>[4x]MSNEIPKPVAPAPDILRCAYAELVVTDLAKSRNFYVDVLGLHVSYEDENQIYLRSFEEFIHHNLVLTKGPVAALKAMAFRVRTPEDVDKAEAYYQELGCR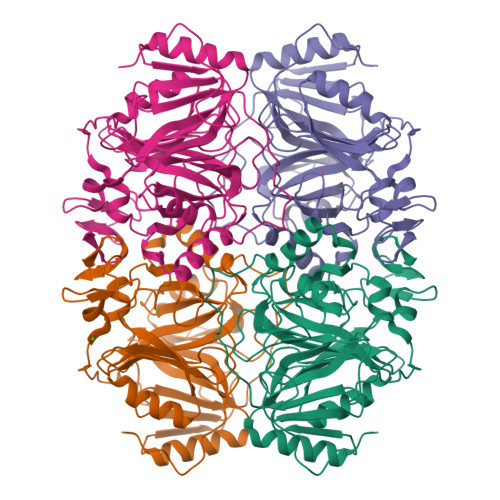TERRKDGFVKGIGDALRVEDPLGFPYEFFFETTHVERLHMRYDLYSAGELVRLDHFNQVTPDVPRGRKYLEDLGFRVTEDIQDDEGTTYAAWMHRKGTVQDTALTGGNGPRLHHVAFSTHEKHNIIQICDKMGALRISDRIERGPGRHGVSNAFYLYILDPDNHRIEIYTQDYYTGDPDNPTITWNVHDNQRRDWWGNPVVPSWYTEASKVLDLDGNVQEIIERTDDSELEVTIGADGFSFTRAGDEDGSYHGQASKGFKLGNQL> MAQASSTPAVSPRPRPRYREERTLVRKLLPRPGQSKQEFRENVKKLRKAFLQFNADVSGVCQWAIQFRPRYGKPAEPTETFWKFFLEPETSLPPNDSRSPEFRRLQAFEAAAGINGAAALDDPAFTNELRDSILAVASRPKTKEAQRLFSRLKDYQPAHRMILAKVAAEWIESRYRRAHQNWERNYEEWKKEKQEWEQNHPELTPEIREAFNQIFQQLEVKEKRVRICPAARLLQNKDNCQYAGKNKHSVLCNQFNEFKKNHLQGKAIKFFYKDAEKYLRCGLQSLKPNVQGPFREDWNKYLRYMNLKEETLRGKNGGRLPHCKNLGQECEFNPHTALCKQYQQQLSSRPDLVQHDELYRKWRREYWREPRKPVFRYPSVKRHSIAKIFGENYFQADFKNSVVGLRLDSMPAGQYLEFAFAPWPRNYRPQPGETEISSVHLHFVGTRPRIGFRFRVPHKRSRFDCTQEELDELRSRTFPRKAQDQKFLEAARKRLLETFPGNAEQELRLLAVALGTDSARAAFFIGKTFQQAFPLKIVKIEKLYEQWPNQKQAGDRRDASSKQPRPGLSRDHVGRHLQKMRAQASEIAQKRQELTGTPAPETTTDQAAKKATLQPFDLRGLTVHTARMIRDWARLNARQIIQLAEENQVDLIVLESLRGFRPPGYENLDQEKKRRVAFFAHGRIRRKVTEKAVERGMRVVTVPYLASSKVCAECRKKQKDNKQWEKNKKRGLFKCEGCGSQAQVDENAARVLGRVFWGEIELPTAIP

Cas12g is an endonuclease belonging to the type V RNA-guided CRISPR–Cas family. However, while most known type V effectors use this domain to cleave DNA substrates, Cas12g, the Cas effector of the newly identified type V-G systems, stands out by exhibiting RNA-guided ribonuclease (RNase) activity instead of cleaving DNA substrates. Cas12g, which is a thermostable protein identified from a hot spring metagenome locus, functions as an RNA-guided ribonuclease (RNase). Cas12g adopts a bilobed architecture encompassing recognition (REC) and nuclease (NUC) lobes.

The Cas12g-sgRNA binary complex was formed by incubating the catalytically inactive Cas12g (D513A) mutant with a 139-nucleotide (nt) sgRNA, which was determined by cryo-EM at a resolution of 3.1 Å and showed a clear density map. The sgRNA used in the complex was generated by fusing a 45-nt crRNA with a 94-nt tracrRNA. Compared to apo-Cas12g, the REC and NUC lobes in the Cas12g-sgRNA binary complex undergo significant rearrangements, creating a central channel accommodating the sgRNA guide region. In the Cas12g-sgRNA complex, the sgRNA is bound to the outer concave surface formed by the Helical 1, Helical 2 and WED domains, which establishes extensive charged interactions. The 3’-end nucleotides A (-3)-A (+1) of crRNA are guided from this outer concave surface into the positively charged central channel through an opening between the WED and Helical 2 domains. The short R:AR duplex 2 is located at the entrance of the central channel and forms extensive hydrogen bonds with residues from the Helical 2 and RuvC domains. Additionally, the short Nuc domain, consisting of 36 aa and containing a CCCC-type zinc finger, is visible in the binary complex and was found to be inserted between the RuvC-II and RuvC-III subdomains. Additionally, a third zinc finger motif, the CCCC-type zinc finger (Cys711-Cys714-Cys735-Cys738), is clearly observed in the Nuc domain of the Cas12g binary complex and coordinates the Zn2+C ion. Although the remaining electron density of the Helical 1 subdomain II region (aa 232–355) that contains these two zinc finger motifs cannot be traced in the binary complex, the orientation can be unambiguously discerned using unsharpened density maps. Specifically, the region spanning aa 232–355 region of the Helical 1 subdomain II, which is positioned away from the core of apo-Cas12g, swings toward the central channel of the binary complex.>MQWSGARALEALLTVAGELRGPPLQLDTGQLLKIAKRGGVTAVEAVHAWRNALTGAPLNLTPEQVVAIASHDGGKQALETVQRLLPVLCQAHGLTPQQVVAIASHDGGKQALETVQRLLPVLCQAHGLTPEQVVAIASHDGGKQALETVQALLPVLCQAHGLTPEQVVAIASNGGGKQALETVQRLLPVLCQAHGLTPQQVVAIASNGGGKQALETVQRLLPVLCQAHGLTPQQVVAIASNGGGKQALETVQRLLPVLCQAHGLTPQQVVAIASNEGGKQALETVQRLLPVLCQAHGLTPQQVVAIASNGGGKQALETVQRLLPVLCQAHGLTPQQVVAIASHDGGKQALETVQRLLPVLCQAHGLTPEQVVAIASNGGGKQALETVQRLLPVLCQAHGLTPEQVVAIASHDGGKQALETVQRLLPVLCQAHGLTPQQVVAIASNGGGRPALESIVAQLSRPDPALAALTNDHLVALACLGGRPALDAVKKLEHHHHHH[2x]

Transcription activator-like (TAL) effectors specifically bind to double stranded (ds) DNA through a central domain of tandem repeats. Each TAL effector (TALE) repeat comprises 33–35 amino acids and recognizes one specific DNA base through a highly variable residue at a fixed position in the repeat. The crystal structures of TAL effector (TALE) proteins bound to their respective target DNAs have revealed that the residue at position 13 is the only one directly involved in DNA base recognition, whereas the 12th residue stabilizes the proper loop conformation. dHax3, an engineered TALE protein, proved to be a useful scaffold for structural characterizations. We then present fifteen crystal structures of engineered dHax3 variants in complex with target DNA molecules, which elucidate the structural basis for the recognition of bases adenine (A) and guanine (G) by reported or uncharacterized TALE codes.

To test this speculation, we generated dHax3 variants with the 34th residue on repeat 7 substituted with different amino acids. In total, we obtained nine high-quality structures that elucidate the accommodation of base A by Leu, Met, Cys, Pro, Trp, His, Thr, Asn, and Glu at the 34th position. On the other hand, Asn34 and Glu34 can both be H-bonded to base A, although the recognition between Glu34 and base A was unreported previously.>GATLSMRPAPIPIEDPEWRQTPPPVSATSGTFRLRRGSRFTWRKECLAVMESYFNENQYPDEAKR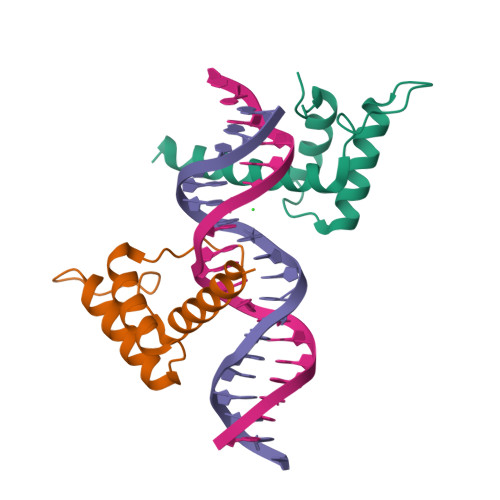EEIANACNAVIQKPGKKLSDLERVTSLKVYNWFANRRKEIKRRANIEA[2x]GLYCYL-L-ALPHA-AMINO-EPSILON-PIMELYL-D-ALANINE | C12 H21 N3 O6 | 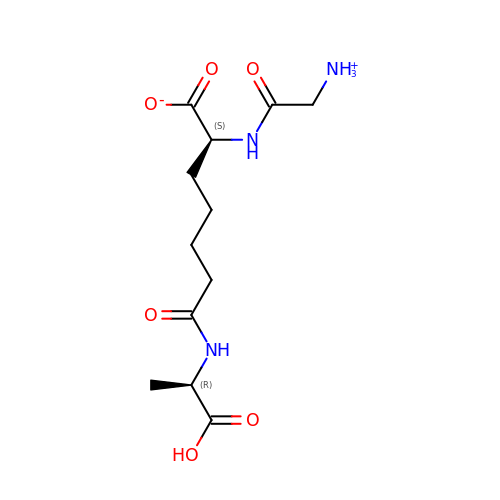ZMQJQOKNTYQVHO-SFYZADRCSA-N Langerhans cells are characterized by the presence of langerin (CD207), a C-type lectin that can act as a pathogen receptor by binding to surface glycoconjugates of microorganisms. Langerin has an extracellular region that contains (1) a C-type carbohydrate-recognition domain (CRD) that binds sugars and (2) a neck region that mediates the formation of trimers. As in other C-type lectins, the CRD of langerin contains a conserved Ca2+ binding site that binds to carbohydrates. Here we report the identification of additional glycan ligands for langerin through screening of a microarray of bacterial lipopolysaccharides and high-resolution crystal structures of the langerin CRD bound to carbohydrates representing a spectrum of ligands.

In order to investigate the potential modes of binding of langerin to both eukaryotic and prokaryotic mannose-containing sugars, we determined the crystal structures for the monomeric full-length langerin CRD bound to various mannose-containing oligosaccharides. For both ligand complexes, electron density was observed in the conserved Ca2+ site in each of the four crystallographically independent copies of the CRD and was fitted with a mannose. In each copy, mannose binds with the 3-OH group interacting with the Ca2+ ligands Glu293 and Asn307, while the 4-OH group interacts with Glu285 and Asn287, which are part of the EPN motif. In this orientation, the axial 2-OH group forms a hydrogen bond with Lys299. In all of the Man4 complexes, as well as in most of the copies of the Man5 complex, only a single-mannose residue is visible, and it cannot be determined whether this corresponds to a particular mannose residue present in these ligands. However, in one copy of the CRD–Man5 complex, there is additional electron density that is best interpreted as an α1–3-linked mannose. Moreover, there is weak density emerging from the anomeric oxygen of this second sugar. These observations indicate that the mannose residue in the primary binding site corresponds to the outer α1–3-linked mannose residue at the nonreducing end of the Man5 oligosaccharide, consistent with the suggestion that langerin can bind to mannose residues at the nonreducing termini of branched structures.

>[4x]QVVSQGWKYFKGNFYYFSLIPKTWYSAEQFCVSRNSHLTSVTSESEQEFLYKTAGGLIYWIGLTKAGMEGDWSWVDDTPFNKVQSARFWIPGEPNNAGNNEHCGNIKAPSLQAWNDAPCDKTFLFICKRPYVPSEP>[2x]GMKVPEAAISRLITYLRILEELEAQGVHRTSSEQLGELAQVTAFQVRKDLSYFGSYGTRGVGYTVPVLKRELRHILGLNRKWGLCIVGMGDLGSA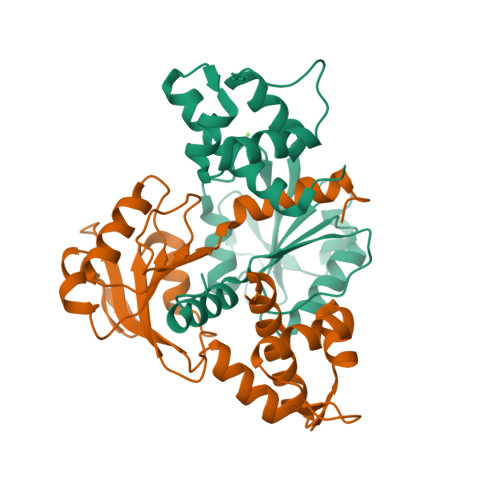LADYPGFGESFELRGFFDVDPEKVGRPVRGGVIEHVDLLPQRVPGRIEIALLTVPREAAQKAADLLVAAGIKGILNFAPVVLEVPKEVAVENVDFLAGLTRLSFAILNPKWR>[2x]GSSHHHHHHMNSKQLIQEAIEARKQAYVPYSKFQVGAALLTQDGKVYRGCNVENASYGLCNCAERTALFKAVSEGDKEFVAIAIVADTKRPVPPC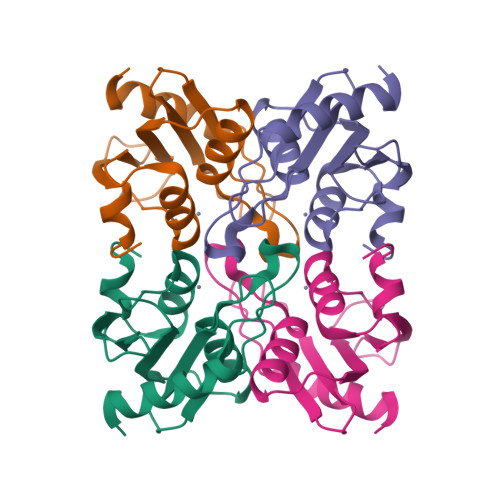GACRQVMVELCKQDTKVYLSNLHGDVQETTVGELLPGAFLAEDLHE> MGYFELQLSALRNVNGELLSGACCDGDGRTTRAGGCGHDECDTYVRVCLKEYQAKVTPTGPCSYGHGATPVLGGNSFYLPPAGAAGDRARARARAGGDQDPGLVVIPFQFAWPRSFTLIVEAWDWDNDTTPNEEL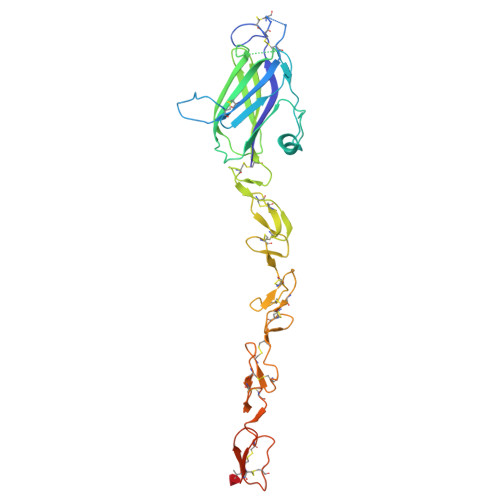LIERVSHAGMINPEDRWKSLHFSGHVAHLELQIRVRCDENYYSATCNKFCRPRNDFFGHYTCDQYGNKACMDGWMGKECKEAVCKQGCNLLHGGCTVPGECRCSYGWQGRFCDECVPYPGCVHGSCVEPWQCNCETNWGGLLCDKDLNYCGSHHPCTNGGTCINAEPDQYRCTCPDGYSGRNCEKAEGSHHHHHHHH>[2x]MNKDIATPIRTKEILKKYGFSFKKSLGQNFLIDTNILNRIVDHAEVTEKTGVIEIGPGIGALTEQLAKRAKKVVAFEIDQRLLPILKDTLSPYE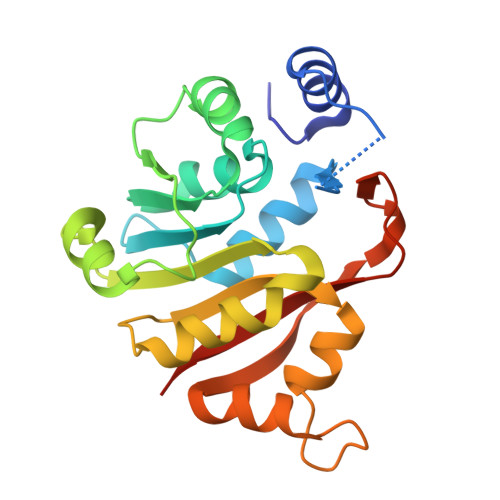NVTVIHQDVLKADVKSVIEEQFQDCDEIMVVANLPYYVTTPIIMKLLEEHLPLKGIVVMLQKEVAERMAADPSSKEYGSLSIAVQFYTEAKTVMIVPKTVFVPQPNVDSAVIRLILRDGPA> MKTQVAIIGAGPSGLLLGQLLHKAGIDNVILERQTPDYVLGRIRAGVLEQGMVDLLREAGVDRRMARDGLVHEGVEIAFAGQRRRIDLKRLSGGKTVTVYGQTEVTRDLMEAREACGATTVYQAAEVRLHDLQGERPYVTFERDGERLRLDCDYIAGCDGFHGISRQSIPAERLKVFERVYPFGWLGLLADTPPVSHELIYANHPRGFALCSQRSATRSRYYVQVPLTEKVEDWSDERFWTELKARLPAEVAEKLVTGPSLEKSIAPLRSFVVEPMQHGRLFLAGDAAHIVPPTGAKGLNLAASDVSTLYRLLLKAYREGRGELLERYSAICLRRIWKAERFSWWMTSVLHRFPDTDAFSQRIQQTELEYYLGSEAGLATIAENYVGL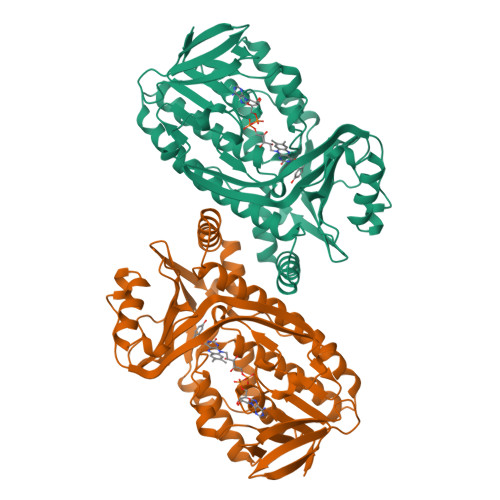PYEEIE> MAESVHLYLKANGSDIKGDSTQTSLGRADSIECVAYSQKVFTAREAGSGLATGRRQYEGIEITKRIDKSSPLLMKALCENQVIDATFKFFRPNPTGDGTTEQFYTVSI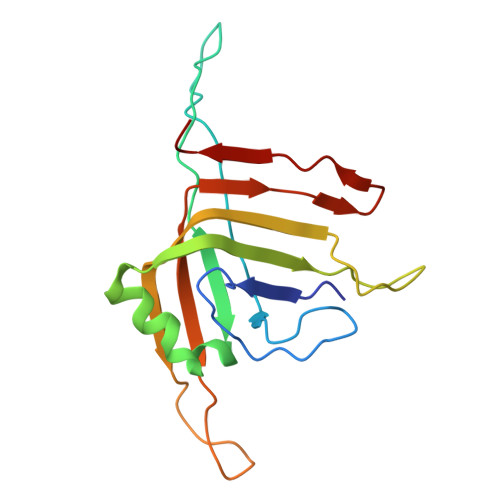KKARINAIQQTVPNSFVPASTNLPPMETLQLVFHTINWTITQGGVTHEDTWDTQR HYDROXYFLUTAMIDE | C11 H11 F3 N2 O4 | 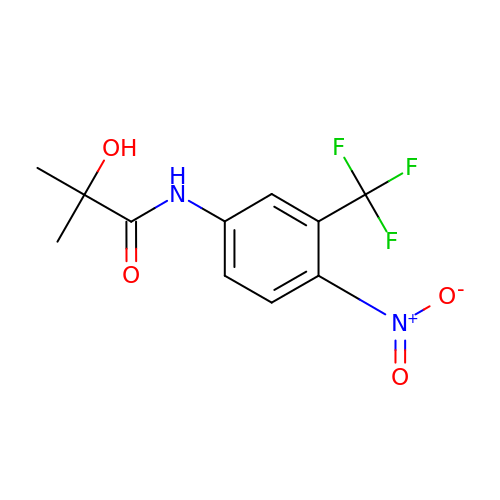YPQLFJODEKMJEF-UHFFFAOYSA-N> MPHLENVVLCRESQVSILQSLFGERHHFSFPSIFIYGHTASGKTYVTQTLLKTLELPHVFVNCVECFTLRLLLEQILNKLNHLSSSEDGCSTEITCETFNDFVRLFKQVTTAENLKDQTVYIVLDKAEYLRDMEANLLPGFLRLQELADRNVTVLFLSEIVWEKFRPNTGCFEPFVLYFPDYSIGNLQKILSHDHPPEYSADFYAAYINILLGVFYTVCRDLKELRHLAVLNFPKYCE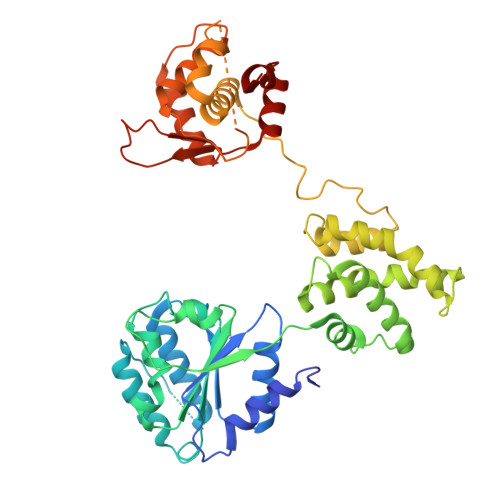PVVKGEASERDTRKLWRNIEPHLKKAMQTVYLREISSSQWEKLQKDDTDPGQLKGLSAHTHVELPYYSKFILIAAYLASYNPARTDKRFFLKHHGKIKKTNFLKKHEKTSNSLLGPKPFPLDRLLAILYSIVDSRVAPTANIFSQITSLVTLQLLTLVGHDDQLDGPKYKCTVSLDFIRAIARTVNFDIIKYLYDFL>SNADRRYKWQTVVSEQLVGAGFNEILNNSLTAGSYYEGLKSHPREMAVELMNPLSQELNCMRQTLLFGGLETLSHNLRRKHLSLYLFEWGKCYRFHAAKRTDETPLAAYAEDDRLGIWICGQRVHNSWAHPEEPTSVFELKAVVEQVLCRVGIETGAYTLKTADNDLYASAMEVKTRSGKLLGTFGTVSTELIKRFEIEQPVYFAELLWDA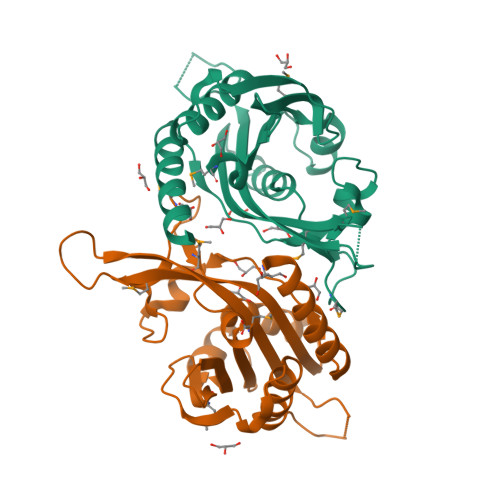LM[2x]2-(methylamino)-1H-benzimidazole-5-carbohydrazide | C9 H11 N5 O | 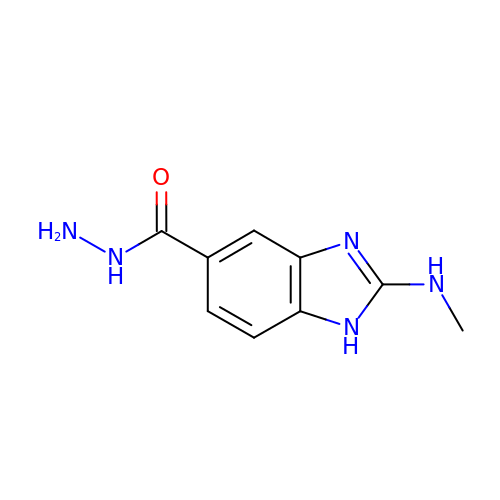UAYYHYYNSIPFPB-UHFFFAOYSA-N CHLORAMPHENICOL | C11 H12 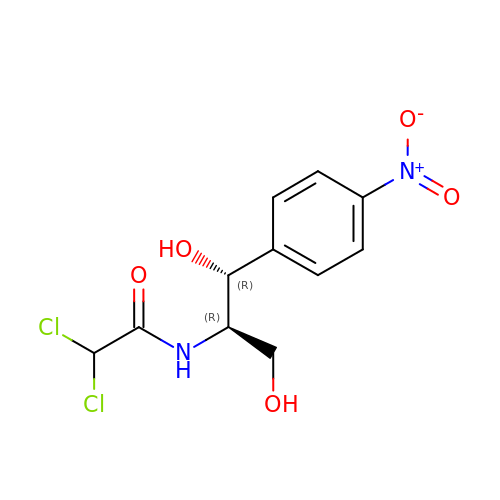Cl2 N2 O5 | WIIZWVCIJKGZOK-RKDXNWHRSA-N> MNNNKAEADTSSSMADPETRPTYTTHHLAIPSGVTQDEFDELKQSVVEFHTYQLSQNQCSSLLAQRIRAPNDVVWSIVRRFDQPQTYKHFIKSCSVSDNFTMAVGSTRDVNLISGLPAATSTERLDILDDDRQVLGISIIGGEHRLRNYRSVISVHGFNRDGAICTVALESYVVDVPEGNTEEDTRLFADTVVKLNLQKLVSVAESQVI;> RSVYELDCIPLWGVVSIQGNRSEMEDAFAVSPHFLKLPIKMLMGDHEGMSPSLTHLTGHFFGVYDGHG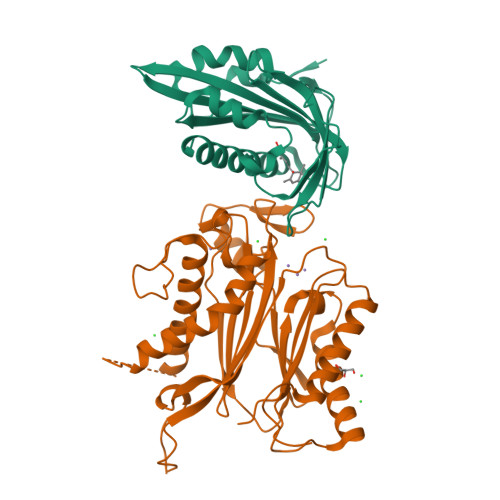GHKVADYCRDRLHFALAEEIERIKDELCKRNTGAGRQVQWDKVFTSCFLTVDGEIEGKIGRAVVGSSDKVLEAVASETVGSTAVVALVCSSHIVVSNCGDSRAVLFRGKEAMPLSVDHKPDREDEYARIENAGGKVIQWQGARVFGVLAMSRSIGDRYLKPYVIPEPEVTFMPRSREDECLILASDGLWDVMNNQEVCEIARRRILMWHKKNGAPPLAERGKGIDPACQAAADYLSMLALQKGSKDNISIIVIDLKAQRKFKTRT> GPETGNKYIEKRAIDLSRERD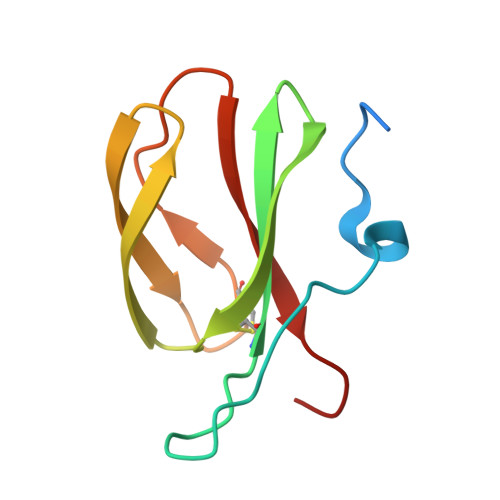PNFFDHPGIPVPECFWFMFKNNVRQDAGTCYSSWKMDMKVGPNWVHIKSDDNCNLSGDFPPGWIVLGKKRPGF>GPLGSMPGEEEERAFLVAREELASALRRDSGQAFSLEQLRPLLASSLPLAARYLQLDAARLVRCNAHGEPRNYLNTLSTALNILEKYGRNLLSPQRPRYWRGVKFNNPVFRSTVDAVQGGRDVLRLYGYTEEQPDGLSFPEGQEEPDEHQVATVTLEVLLLRTELSLLLQNTHPRQQALEQLLE[2x];>[2x]DPAIVQCAWAALYCDMQ

To target disease-causing proteins that are inaccessible to small-molecule or antibody therapies, we are exploring the use of a nature-inspired drug modality that exploits the intrinsically favorable properties of synthetically constrained α-helical polypeptides (Helicons). Here, we report a rapid, high-throughput screening platform utilizing phage display that enables an unbiased mapping of the α-helical interactome of a given protein without any prior knowledge of its structure or known binding partners. Analysis of 14 high-resolution crystal structures of Helicon–protein complexes across six different protein domains reveals a range of binding modes, all of which are “side-on”, i.e., mediated exclusively by Helicon side-chains rather than involving main chain amide interactions. Biochemical and structural experiments demonstrate diverse functional impacts by the Helicons which bind these sites, including inhibition of protein–protein interactions, inhibition of enzymatic activity, induced conformational rearrangement, and induced dimerization.

We began with the E3 ubiquitin ligase RNF31, which is an integral component of the linear ubiquitin chain assembly complex. RNF31 is a 1,072-amino acid protein comprised of multiple folded and disordered regions. We screened two of the nonenzymatic folded domains, the PUB and UBA domains, each at multiple concentrations and in the presence or absence of a known binding partner. Most hits for the RNF31 PUB domain could be grouped into two families of related clusters (C41 to C43 and C44 to C45), both of which competed with the natural binding partner Otulin, and both of which appeared to contain a critical tyrosine residue – also found in Otulin – but that had otherwise dissimilar logos. Upon solving X-ray cocrystal structures of member from a representative cluster of each family, we found that two Helicons, FP06649 from Cluster C44 and FP06652 from C41, bound the same site at the protein surface, but that they engaged this site using completely different binding modes, with the critical tyrosine residues oriented differently. This observation was our first structural evidence of the ability of Helicons to identify distinct binding solutions to a common site, which we have since observed for several other target proteins.> GSVDIEVQDLEEFALRPAPQGITIKCRITR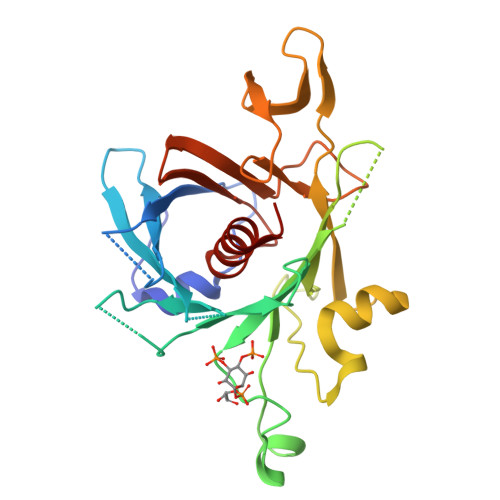DKKGMDRGMFPTYFLHLDREDGKKVFLLAGRKRKKSKTSNYLISVDPTDLSRGGDSYIGKLRSNLMGTKFTVYDNGVNPQKASSSTLESGTLRQELAAVCYETNVLGFKGPRKMSVIVPGMNMVHERVCIRPRNEHETLLARWQNKNTESIIELQNKTPVWNDDTESYVLNFHGRVTQASVKNFQIIHGNDPDYIVMQFGRVAEDVFTMDYNYPLCALQAFAIALSSFDSKLACE>[2x]GMDMKTKLQTIIGMFQITAWDETSYFESDNGAKLTQAVITQSYQ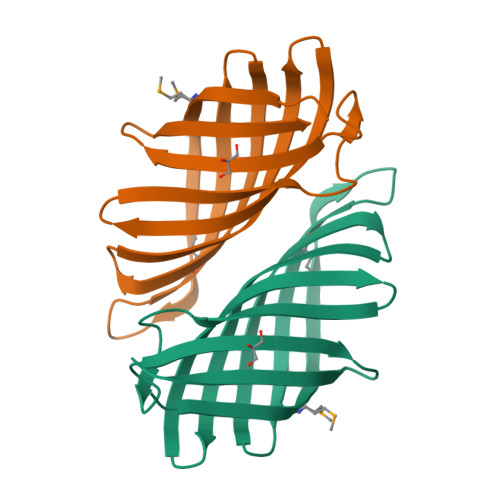GVLQGHSEIRYLMSYQDNANATFVGFEHFTGSLGDKKGSFILQHKGLFAAGVASSEFELVERSATGDFVHLVGKGHFVSTENGQANYQITLQDS> GSDDLNVKGLVLATVSKINYKYQSVEVKVNNLTLGSRIGDDGSLAVPYPKSFIGRTPEGSVFGTKPLITEGSVVLIGFLNDDINSPIILSVYGDNEQNKMINTNPLDGGKFDTESVYKYSSSLYEILPSLNYKYDDGEGTSIRTYNGKSFFSMTSGEEEKPQATDFYTGTEYQDLFTSYYGNKTLIEPRIQKAPNMLFKHQGVFYDDGTPDNHITTLFISERGDIRASVLNTETQKRTTQEMSSDGSYRVIKQDDDLMLDEAQVWIEYGISEDNKFYIKNDKHKFEFTDEGIYIDDKPMLENLDESIAEAMKNLNEIQKELDDINYLLKGVGKDNLEELIESTKESIEASKKATSDVNRLTTQIAEVSGRTEGIITQFQKFRDETFKDFYEDASTVINEVNQNFPTMKTDVKTLKTKVDNLEKTEIPNIKTRLTELENNNNNADKIISDRGEHIGAMIQLEENVTVPMRKYMPIPWSKVTYNNAEFWDSNNPTRLVVPKGITKVRVAGNVLWDSNATGQRMLRILKNGTYSIGLPYTRDVAISTAPQNGTSGVIPVKEGDYFEFEAFQDSEGDRQFRADPYTWFSIEAIELETETMEKDFMLIGHRGATGYTDEHTIKGYQMALDKGADYIELDLQLTKDNKLLCMHDSTIDRTTTGTGKVGDMTLSYIQTNFTSLNGEPI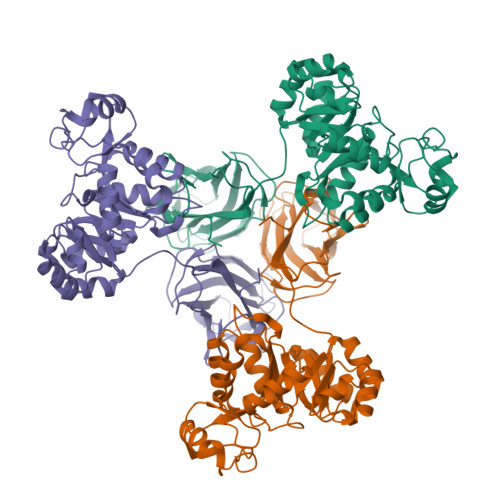PSLDDVLNHFGTKVKYYIETKRPFDANMDRELLTQLKAKGLIGIGSERFQVIIQSFARESLINIHNQFSNIPLAYLTSTFSESEMDDCLSYGFYAIAPKYTTITKELVDLAHSKGLKVHAWTVNTKEEMQSLIQMGVDGFFTNYLDEYKKI> HHHHHHQEEDLPRPSISAEPGTVIPLGSHVTFVCRGPVGVQTFRLERESRSL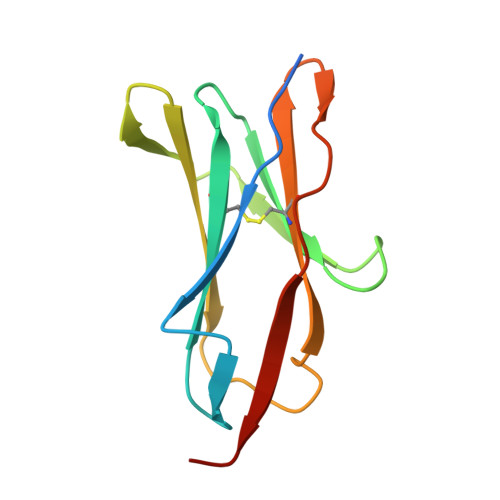YSDTEDVSQTSPSESEARFRIDSVSEGNAGPYRCIYYKPPKWSEQSDYLELLVKEAAA> MGHHHHHHHHHHSSGHIDDDDKHMIKLSNITKVFHQGTRTIQALNNVSLHVPAGQIYGVIGAS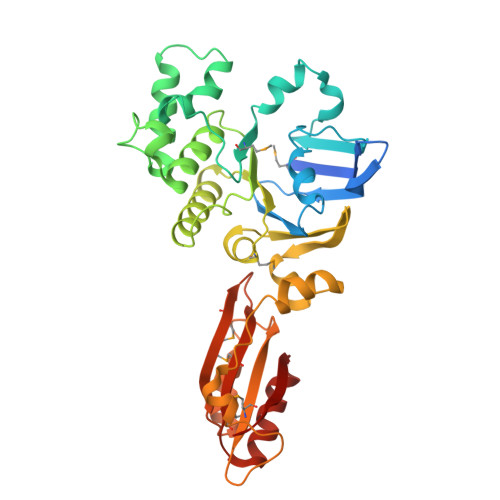GAGKSTLIRCVNLLERPTEGSVLVDGQELTTLSESELTKARRQIGMIFQHFNLLSSRTVFGNVALPLELDNTPKDEVKRRVTELLSLVGLGDKHDSYPSNLSGGQKQRVAIARALASNPKVLLCDQATSALDPATTRSILELLKDINRRLGLTILLITHEMDVVKRICDCVAVISNGELIEQDTVSEVFSHPKTPLAQKFIQSTLHLDIPEDYQERLQAEPFTDCVPMLRLEFTGQSVDAPLLSETARRFNVNNNIISAQMDYAGGVKFGIMLTEMHGTQQDTQAAIAWLQEHHVKVEVLGYV5-chloranyl-N-[2-(3-methoxyphenyl)ethanimidoyl]-2-piperidin-4-yloxy-benzamide | C21 H24 Cl 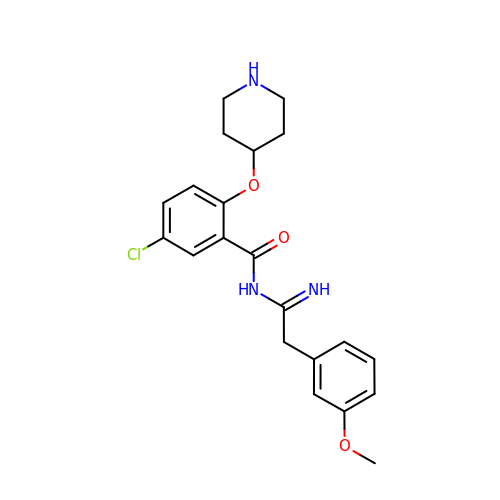N3 O3 | ASGVJWYYPPACHP-UHFFFAOYSA-N>TTNPVDLWSAPSSQARLEKEYFDQHFGPFFRTEQLIIRAPLTDKHIYQPYPSGADVPFGPPLDIQILHQVLDLQIAIENITASYDNETVTLQDICLAPLSPYNTN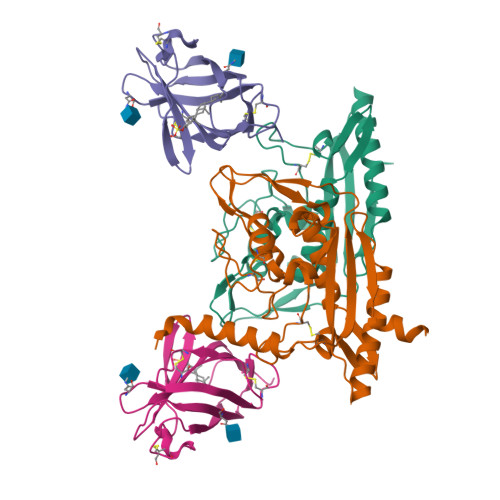CTILSVLNYFQNSHSVLDHKKGDDFFVYADYHTHFLYCVRAPASLNDTSLLHDPCLGTFGGPVFPWLVLGGYDDQNYNNATALVITFPVNNYYNDTEKLQRAQAWEKEFINFVKNYKNPNLTISFTAERSIEDELNRESDSD[2x];>[2x]EPVQFKDCGSVDGVIKEVNVSPCPTQPCQLSKGQSYSVNVTFTSNIQSKSSKAVVHGILMGVPVPFPIPEPDGCKSGINCPIQKDKTYSYLNKLPVKSEYPSIKLVVEWQLQDDKNQSLFCWEIPVQIVSHLA> NECISVKGRIYSILKQIGSGGSSKVFQVLNEKKQIYAIKYVNLEEADNQTLDSYRNEIAYLNKLQQHSDKIIRLYDYEITDQYIYMVMECGNIDLNSWLKKKKSIDPWERKSYWKNMLEAVHTIHQHGIVHSDLKPANFLIVDGMLKLIDFGIANQMQPDTTSVVKDSQVGTVNYMPPEAIKDMSSSRENGKSKSKISPKSDVWSLGCILYYMTYGKTPFQQIINQISKLHAIIDPNHEIEFPDIPEKDLQDVLKCCLKRDPKQRISIPELLAHPYVQIQTHPVNQMAKGTTEEMKYVLGQLVGLNSPNSILKAAKTLYEHYSGGESHNSSSSKTFEKKR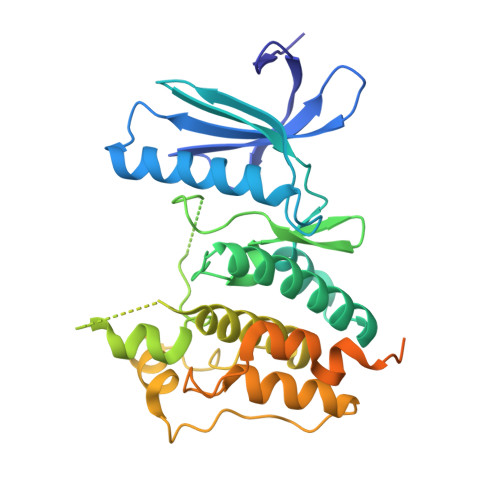GKK(1~{R})-1-cyclohexyl-2-pyrido[3,4-b]indol-9-yl-ethanol 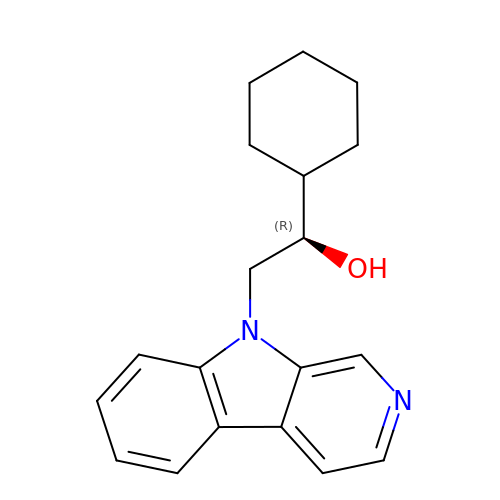| C19 H22 N2 O | MMCCSFCZNUXGJD-IBGZPJMESA-N>[6x]MGHHHHHHMSADDDVAYVVDMLRKSR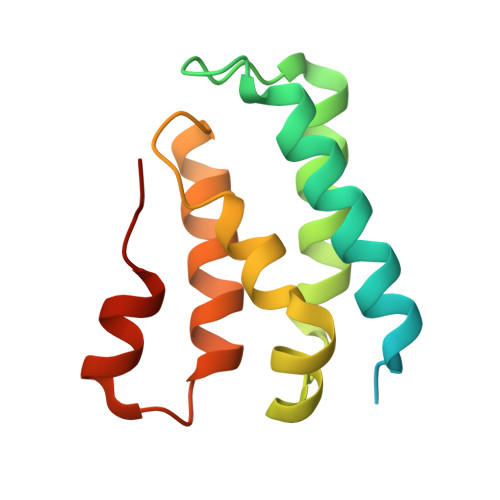HDVTNATLETTGKELTETYMECLNGDVVEVSIANEERIVSLLSSLASANVTLKQLIGTKIGVAVGQFLSDGFPPHIVRFSKGILDYWFRQLPEEVQKQLLAKRALGT> RTSTIMTDYNPNYSFAGKTSSISDLKEVPRKNITLIRGLGHGAFGEVYEGQVSGMPNDPSPLQVAVKTLPE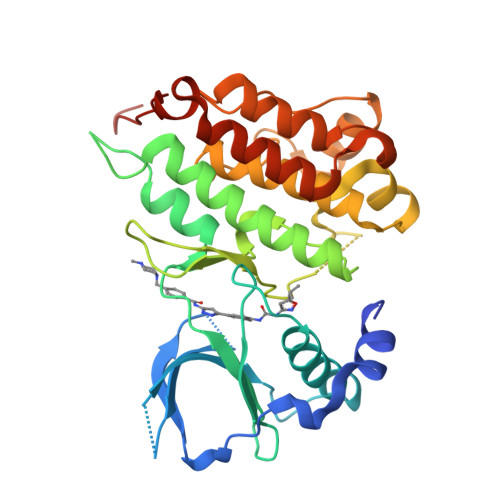VCSEQDELDFLMEALIISKFNHQNIVRCIGVSLQSLPRFILLELMAGGDLKSFLRETRPRPSQPSSLAMLDLLHVARDIACGCQYLEENHFIHRDIAARNCLLTCPGPGRVAKIGDFGMARDIYRASYYRKGGCAMLPVKWMPPEAFMEGIFTSKTDTWSFGVLLWEIFSLGYMPYPSKSNQEVLEFVTSGGRMDPPKNCPGPVYRIMTQCWQHQPEDRPNFAIILERIEYCTQDPDVINTALPIEYGPLVEEEEK> MKQGLQLRLSQQLAMTPQLQQAIRLLQLSTLELQQELQQALESNPLLEQTDLHDEVEAKEVEDRESLDTVDALEQKEMPDELPLDASWDEIYTAGTPSGNGVDYQDDELPVYQGETTQTLQDYLMWQVELTPFTDTDRAIATSIVDAVDDTGYLTIQIEDIVDSIGDDEIGLEEVEAVLKRIQRFDPVGVAAKDLRDCLLIQLSQFAKETPWLEEARLIISDHLDLLANHDFRTLMRVTRLKEEVLKEAVNLIQSLDPRPGQSIHTSEPEYVIPDVLVRKVSGRWTVELNADSI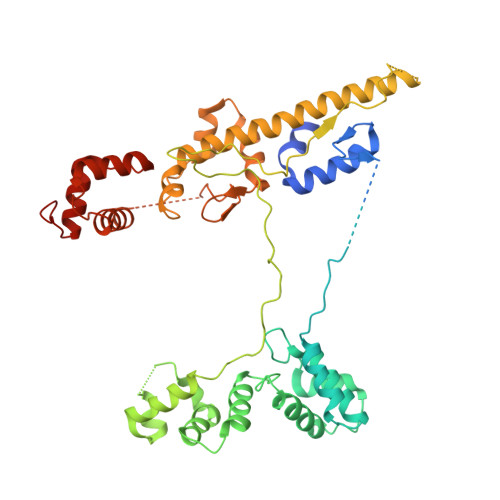PRLKINQQYAAMGNSARNDADGQFIRSNLQEARWLIKSLESRNDTLLRVSRCIVEQQQAFFEQGEEYMKPMVLADIAQAVEMHESTISRVTTQKYLHSPRGIFELKYFFSSHVNTEGGGEASSTAIRALVKKLIAAENPAKPLSDSKLTSMLSEQGIMVARRTVAKYRESLSIPPSNQRKQLV> GQKTENKTEMSIQNS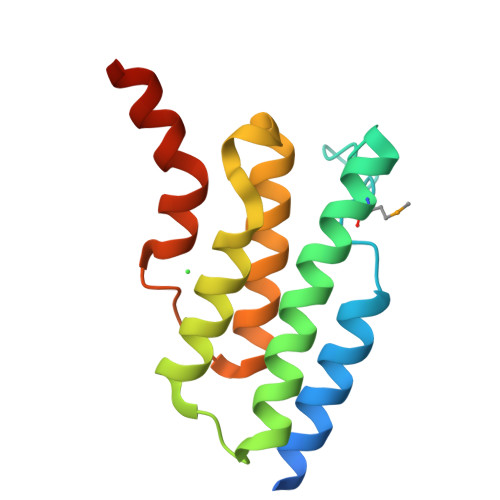NSIVIQQLEKFKAQDHFAGDGQLYTGVQNSALRMSLNQKVADTAQAFIALYQQKNEPTKAELLQVLANGISQIDPDKLDTEDREQVATTFESFLDIVGLESSEGILNKWVYGEEISKLLEQDKH>GSLHMSFETRFEKMDNLLRDPKSEVNSDCLLDGLDALVYDLDFPALRKNKNIDNFLSRYKDTINKIRDLRMKAEDYEVVKVIGRGAFGEVQLVRHKSTRKVYAMKLLSKFEMIKRSDSAFFWEERDIMAFANSPWVVQLFYAFQDDRYLYMVMEYMPGGDLVNLMSNYDVPEKWARFYTAEVVLALDAIHSMGFIHRDVKPDNMLLDKSGHLKLADFGTCMKMNKEGMVRCDTAVGTPDYISPEVLKSQGGDGYYGRECDWWSVGVFLYEMLVGDTPFYADSLVGTYSKIMNHKNSLTFPDDNDISKEAKNLICAFLTDREVRLGRNGVEEIKRHLFFKND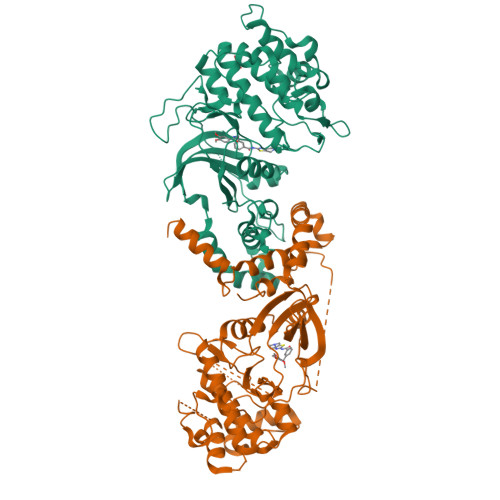QWAWETLRDTVAPVVPDLSSDIDTSNFDDLEEDKGEEETFPIPKAFVGNQLPFVGFTYYSNRRYLSSANPNDNR[4x]>SNAMLDVAIIGGGPAGLSAGLYATRGGLKNVVMFEKGMPGGQITSSSEIENYPGVAQVMDGISFMAPWSEQCMRFGLKHEMVGVEQILKNSDGSFTIKLEGGKTELAKAVIVCTGSAPKKAGFKGEDEFFGKGVSTCATCDGFFYKNKEVAVLGGGDTALEEALYLANICSKIYLIHRRDEFRAAPSTVEKVKKNEKIELITSASVDEVYGDKMGVAGVKVKLKDGSIRDLNVPGIFTFVGLNVRNEILKQDDSKFLCNMEEGGQVSVDLKMQTSVAGLFAAGDLRKDAPKQVICAAGDGAVAALSAMA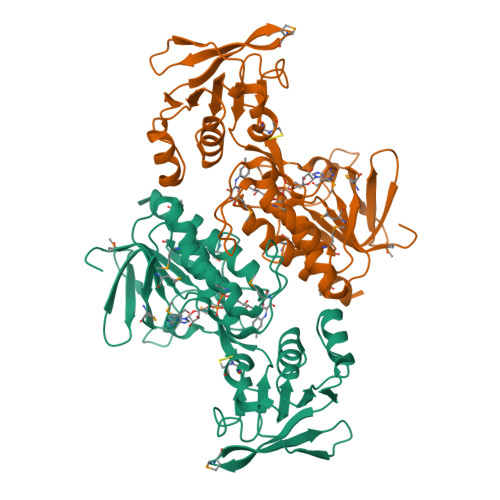YIESLH[2x]> RQLVFLEWHEAPTIAVALLAALGFLSTLAILVIFWRHFQTPIVRSAGGPMCFLMLTLLLVAYMVVPVYVGPPKVSTCLCRQALFPLCFTICISCIAVRSFQIVCAFKMASRFPRAYSYWVRYQGPYVSMAFITVLKMVIVVIGMLATGLSPTTRTDPDDPKITIVSCNPNYRNSLLFNTSLDLLLSVVGFSFAYMGKELPTNYNEAKFITLSMTFYFTSSVSLCTFMSAYSGVLVTIVDLLVTVLNLLAISLGYFGPKCYMILFYPERNTPAYFNSMI;> PRRPKFLAWGEPVVLSLLLLLCLVLGLALAALGLSVHHWDSPLVQASGGSQFCFGLICLGLFCLSVLLFPGRPSSASCLAQQPMAHLPLTGCLSTLFLQAAETFVESELPLSWANWLCSYLRGLWAWLVVLLATFVEAALCAWYLIAFPPEVVTDWSVLPTEVLEHCHVRSWVSLGLVHITNAMLAFLCFLGTFLVQSQPGRYNRARGLTFAMLAYFITWVSFVPLL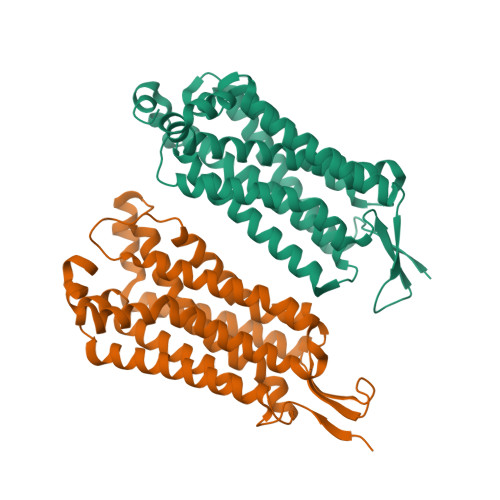ANVQVAYQPAVQMGAILVCALGILVTFHLPKCYVLLWLPKLNTQEFFL>GSMAKVQVNNVVVLDNPSPFYNPFQFEITFECIEDLSEDLEWKIIYVGSAESEEYDQVLDSVLVGPVPAGRHMFVFQADAPNPGLIPDADAVGVTVVLITCTYRGQEFIRVGYYVNNEYTETELRENPPVKPDFSKLQRNILASNPRVTRFHINWED[8x];>EELHSLDPRRQELLEARFTGV[16x]

By binding histone H3–H4 dimers, the histone chaperone ASF1 facilitates nucleosome assembly and turnover and modulates histone post-translational modifications. ASF1 consists of an N-terminal 155-residue immunoglobulin-like domain (ASF1-NT) followed by a presumably unstructured C-terminal tail. As expected from prior structures of human and yeast ASF119,20,59, ASF1a-NT adopted an immunoglobulin (Ig) domain-like fold, composed of a β sandwich topped by α helices. Specifically, phosphorylation of the C-terminal tail of histone-free ASF1 by tousled-like kinases (TLKs) increases its association with the H3–H4 dimer and downstream chaperones, which has been suggested to promote the provision of histones for chromatin assembly.

Apo-ASF1a-NT crystallized in space group C2 with seven molecules in the asymmetric unit, while the complex with the TLK2 peptide crystalized in the P21 space group with eight complexes in the asymmetric unit. The structure of apo-ASF1 NT domain was resolved to 2.1 Å and in complex with the TLK2 peptide to 2.71 Å. Our ASF1a·TLK2 peptide complex structure data contained additional electron density absent from the apo-ASF1a structure, consistent with peptide binding. Surprisingly, additional density was observed at two of the previously characterized binding surfaces, the H3 binding site and at the B-domain binding site. In the ASF1a·TLK2 peptide complex, peptide binding at the H3-binding site is observed in all eight copies of ASF1a-TLK2 residues spanning Asp9 to Gly22 can be built into each copy, with residues His6 to Val23 visible in some cases. The overall mode of interaction is similar to how ASF1a engages helix α3 of histone H3 as seen in ASF1a·H3/H4 structures. The interaction at this interface is mediated by polar contacts between Arg12 and Arg19 of TLK2 (analogous to Lys122 and Arg129 in H3) and ASF1a residues Asp88 and Asp54, respectively. Additional polar contacts are made between the sidechains of ASF1a Arg108 and Thr147 and main chain groups of Arg19 and Phe20 near the C-terminus of the TLK peptide (or Arg129 and Arg131 of H3). Overall, the TLK2 N-terminal peptide binding at this interface does not appear homologous to HIRA, while its binding at the H3 binding site is strikingly similar to what is observed for H3 in terms of sequence, structure and side chain interactions. Our co-crystal structure revealed that the TLK2 N-terminal region strikingly recapitulates a fragment of histone H3 in its interaction with ASF1a, suggesting that TLKs recruit ASF1 by mimicking their chaperone client.> ACRQEPQPQGPPPAAGAVASYDYLVIGGGSGGLESAWRAAELGARAAVVESHKLGGTCVNVGCVPKKVMWNTAVHSEFMHDHADYGFPSCEGKFNWRVIKEKRDAYVSRLNAIYQNNLTKSHIEIIRGHAAFTSDPKPTIEVSGKKYTAPHILIATGGMPSTPHESQIPGASLGITSDGFFQLEELPGRSVIVGAGYIAVEMAGILSALGSKTSLMIRHDKVLRSFDSMISTNCTEELENAGVEVLKFSQVKEVKKTLSGLEVSMVTAVPGRLPVMTMIPDVDCLLWAIGRVPNTKDLSLNKLGIQTDDKGHII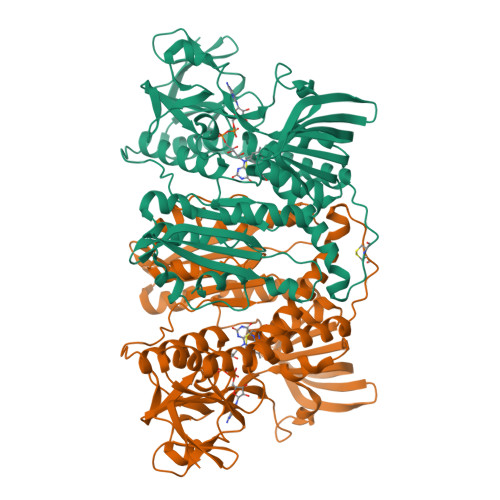VDEFQNTNVKGIYAVGDVCGKALLTPVAIAAGRKLAHRLFEYKEDSKLDYNNIPTVVFSHPPIGTVGLTEDEAIHKYGIENVKTYSTSFTPMYHAVTKRKTKCVMKMVCANKEEKVVGIHMQGLGCDEMLQGFAVAVKMGATKADFDNTVAIHPTSSEELVTLR> MSHPPSNTPPVKPGGLPLLGHILEFGKNPHAFLMALRHEFGDVAEFRMFHQRMVLLTGSQASEAFYRAPDEVLDQGPAYRIMTPIFGRGVVFDARIERKNQQLQMLMPALRDKPMRTYSEIIVA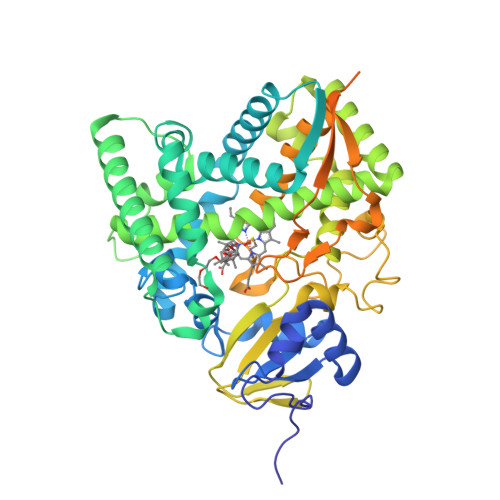EVEAMLRDWKDAGTIDLLELTKELTIYTSSHCLLGAEFRHELNTEFAGIYRDLEMGIQPIAYVFPNLPLPVFKRRDQARVRLQELVTQIMERRARSQERSTNVFQMLIDASYDDGSKLTPHEITGMLIATIFAGHHTSSGTTAWVLIELLRRPEYLRRVRAEIDALFETHGRVTFESLRQMPQLENVIKEVLRLHPPLILLMRKVMKDFEVQGMRIEAGKFVCAAPSVTHRIPELFPNPELFDPDRYTPERAEDKDLYGWQAFGGGRHKCSGNAFAMFQIKAIVCVLLRNYEFELAAAPESYRDDYRKMVVEPASPCLIRYRRRDAPAAVDAKASAGEAPAETLRGAFRVTVDRDLCKGHGNCMAEAPEIFRVDEDGRLTLLSETPDPVLVGAALAAERFCPARAIKILPQRDPATRDRSLSPSGED(5R)-4-(5-bromothiophene-2-carbonyl)-5-(3,5-dimethylphenyl)-7-methyl-1,3,4,5-tetrahydro-2H-1,4-benzodiazepin-2-one 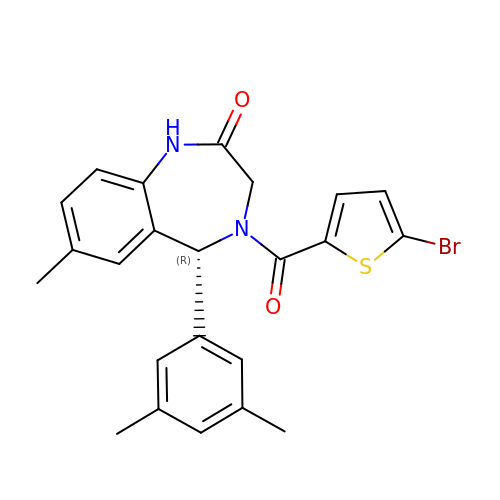| C23 H21 Br N2 O2 S | NIPTUMFVYBXSMZ-JOCHJYFZSA-N> NTGDNSVCTTKTSTRIVGGTESSWGEWPWQVSLQVKLTAQRHLCGGSLIGHQWVLTAAHCFDGLPLQDVWRIYSGILELSDITKDTPFSQIKEIIIHQNYKVSEGNHDIALIKLQAPLEYTEFQK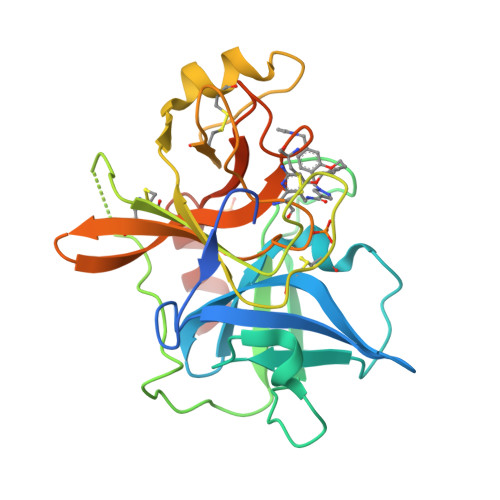PISLPSKGDTSTIYTNCWVTGWGFSKEKGEIQNILQKVNIPLVTNEECQKRYQDYKITQRMVCAGYKEGGKDACKGDSGGPLVCKHNGMWRLVGITSWGEGCARREQPGVYTKVAEYMDWILEKTQSSDGKAQMQSPA> NLINFMEMIRYTIPCEKTWGEYADYGCYCGAGGSGRPIDALDRCCYVHDNCYGDAEKKHKCNPKTQSYSYKLTKRTIICYGAAGTCARIVCD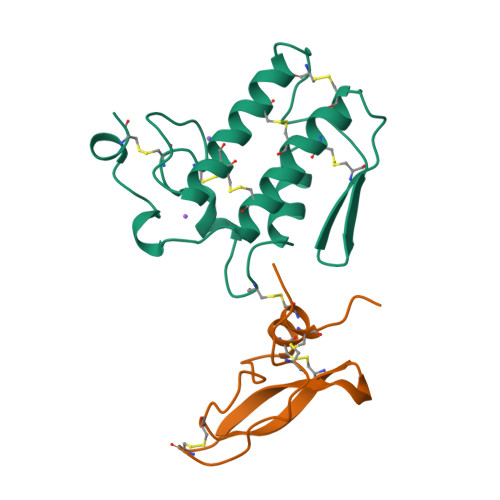CDRTAALCFGNSEYIEGHKNIDTARFCQ;> RKRHPDCDKPPDTKICQTVVRAFYYKPSAKRCVQFRYGGCNGNGNHFKSDHLCRCECLEYR> MMMYIQVLGSAAGGGFPQWNCNCVNCKGYRDGTLKATARTQSSIALSDDGVHWILCNASPDIRAQLQAFAPMQPARALRDTGINAIVLLDSQIDHTTGLLSLREGCPHQVWCTDMVHQDLTTGFPLFNMLSHWNGGLQWNRIELEGSFVIDACPNLKFTPFPLRSAAPPYSPHRFDPHPGDNLGLMVEDTRTGGKLFYAPGLGQVDEKLLAMMHGADCLLVDGTLWEDDEMQRRGVGTRTGREMGHLAQNGPGGTLEVLDGFPRQRKVLIHINNTNPILDENSPERAEVLRRGVEVAFDGMSIE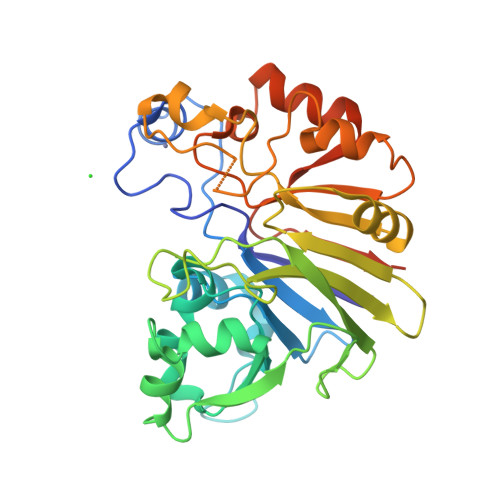LLEHHHHHHLEHHHHHH>[4x]MRIPLVGKDSIESKDIGFTLIHEHLRVFSEAVRQQWPHLYNEDEEFRNAVNEVKRAMQFGVKTIVDPTVMGLGRDIRFMEKVVKATGINLVAGTGIYIYIDLPFYFLNRSIDEIADLFIHDIKEGIQGTLNKAGFVKIAADEPGITKDVEKVIRAAAIANKETKVPIITHSNAHNNTGLEQQRILTEEGVDPGKILIGHLGDTDNIDYIKKIADKGSFIGLDRYGLDLFLPVDKRNETTLRLIKDGYSDKIMISHDYCCTIDIGTAKPEYKPKLAPRWSITLIFEDTIPFLKRNGVNEEVIATIFKENPKKFFS

PLLs are natural lactonases endowed with promiscuous phosphotriesterase activity. The catalytic center contained two metal cations coordinated by four histidines, an aspartic acid and a carboxylated lysine residue. A structural analysis of SsoPox, a hyperthermostable counterpart of the PLL family from Sulfolobus solfataricus, has revealed that loop 7 is shorter in SsoPox than in PTEs; linking the active site to the loop 8, which forms a hydrophobic channel that accommodates AHLs aliphatic chain. Indeed, W263 is located at the start of loop 8, involved in the dimer interface of the enzyme and positions the lactone cycle of the substrate onto the bi-metallic catalytic center.

Noteworthy, subtle changes, such as W263L or W263I, yield to a large tradeoff in catalytic activities. However, whereas detergent-induced flexibility has no effect on the lactonase activity, we isolated variants of W263 that exhibit increased lactonase activities (W263T/V/I). These variants exhibit dramatic improvement of their oxo-lactonase catalytic efficiencies (148-fold for variant W263T), while the activity for the best AHL substrate is compromised (3-oxo-C10 AHL; for the wild-type enzyme). Conversely, the LacSV group dramatically increases oxo-lactonase activity and 3-oxo-C12 AHLase activities, while the phosphotriesterase activity is mildly modulated and 3-oxo-C10 AHLase is decreased. The residues selected in the LacSV group (T, V, I) are overall smaller than those selected in the PteSV group (F, L, M) with the exception of isoleucine (I). The analysis of the normalized B-factors of the variants clearly reveal that the substitution W263 is destabilizing (as confirmed by the Tm of the variants), but also that the active site loops of PteSV are significantly more disordered than those of LacSV. PteSV lose their activity before the loss of the global structure (Tm), whereas LacSV do not, and exhibit a similar thermophilicity profile to that of the wild-type enzyme.>[2x]MKGRLISSDPYRQQFLVERAVSFSHRQRDCSELISVLPRHALQQIDGFGGSFTEGAGVVFNSMSEKTKAQFLSLYFSAQEHNY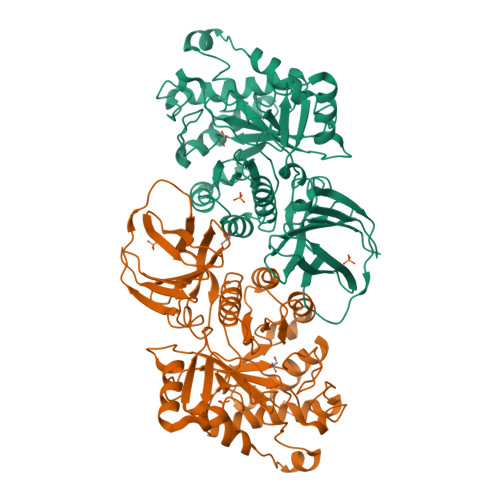TLARMPIQSCDFSLGNYAYVDSSADLQQGRLSFSRDEAHLIPLISGALRLNPHMKLMASPWSPPAFMKTNNDMNGGGKLRRECYADWADIIINYLLEYRRHGINVQALSVQNEPVAVKTWDSCLYSVEEETAFAVQYLRPRLARQGMDEMEIYIWDHDKDGLVDWAELAFADEANYKGINGLAFHWYTGDHFSQIQYLAQCLPDKKLLFSEGCVPMESDAGSQIRHWHTYLHDMIGNFKSGCSGFIDWNLLLNSEGGPNHQGNLCEAPIQYDAQNDVLRRNHSWYGIGHFCRYVRPGARVMLSSSYDNLLEEVGFVNPDGERVLVVYNRDVQERRCRVLDGDKEIALTLPPSGASTLLWRQESI>[6x]MKHLISMKDIGKEEILEILDEARKMEELLNTKRPLKLLEGKILATVFYEPSTRTRLSFETAMKRLGGEVITMTDLKSSSVAKGESLIDTIRVISGYADIIVLRHPSEGAARLASEYSQVPIINAGDGSNQHPTQTLLDLYTIMREIGRIDGIKIAFVGDLKYGRTVHSLVYALSLFENVEMYFVSPKELRLPKDIIEDLKAK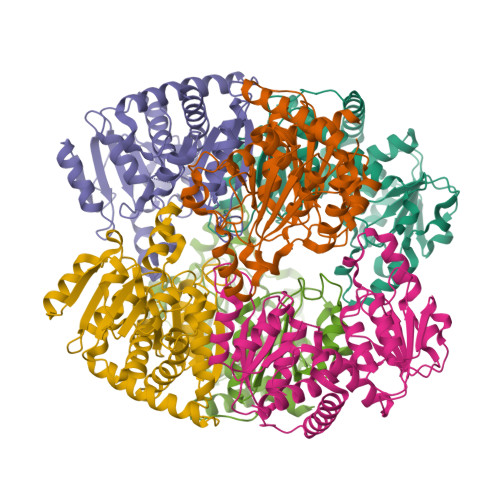NIKFYEKESLDDLDDDIDVLYVTRIQKERFPDPNEYEKVKGSYKIKREYVEGKKFIIMHPLPRVDEIDYDVDDLPQAKYFKQSFYGIPVRMAILKKLIEDNEGE>[2x]GPMGTDWPVYHRIDGPIVMIGFGSIGRGTLPLIERHFAFDRSKLVVIDPSDEARKLAEARGVRFIQQAVTRDNYRELLVPLLTAGPGQGFCVNLSVDTSSLDIMELARENGALYIDTVVEPWLGFYFDPDLKPEARSNYALRETVLAARRNKPGGTTAVSCCG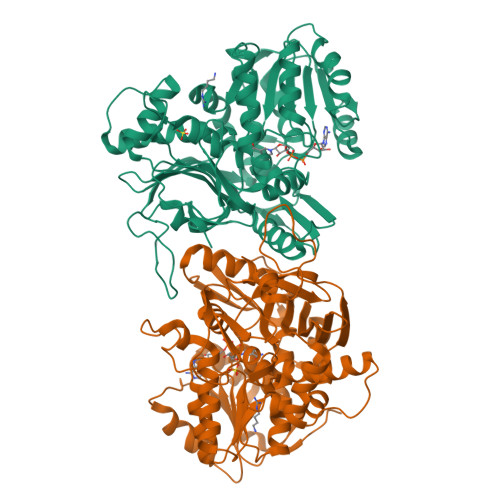ANPGMVSWFVKQALVNLAADLGVTGEEPTTREEWARLAMDLGVKGIHIAQRDTQRASFPKPFDVFVNTWSVEGFVSEGLQPAELGWGTFERWMPDNARGHDSGCGAGIYLLQPGANTRVRSWTPTAMAQYGFLVTHNESISIADFLTVRDAAGQAVYRPTCHYAYHPCNDAVLSLHEMFGSGKRQSDWRILDETEIVDGIDELGVLLYGHGKNAYWYGSQLSIEETRRIAPDQNATGLQVSSAVLAGMVWALENPNAGIVEADDLDFRRCLEVQTPYLGPVVGVYTDWTPLAGRPGLFPEDIDTSDPWQFRNVLVRD> MLKNGMRPIHPGEILREEFQKEMGFSAAALARALGVATPTVNNILRERGGVSADMALRLSICLDTTPEFWLNLQTAFDLRTAEQQHG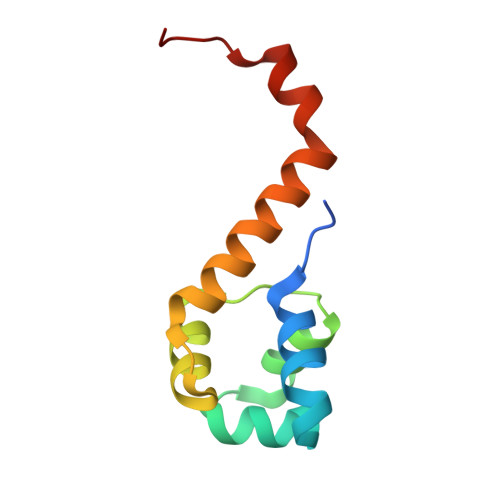DEIIGSVQRLVA>[2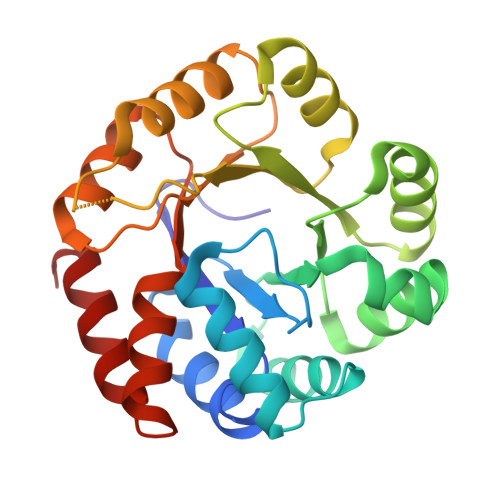x]MFKDGSLIPYLTAGDPDKQSTLNFLLALDEYAGAIELGIPFSDPIADGKTIQESHYRALKNGFKLREAFWIVKEFRRHSSTPIVLMTYYNPIYRAGVRNFLAEAKASGVDGILVVDLPVFHAKEFTEIAREEGIKTVFLAAPNTPAERLKVIDDMTTGFVYLVSLYGTTGAREEIPKTAYDLLRRAKRICRNKVAVGFGVSKREHVVSLLKEGANGVVVGSALVKIIGEKGREATEFLKKKVEELLGI>MAAQNEQRPERIKTTPYLEGDVLSSDSGPLLSVFALQEIMQKVRQVQADYMTATREVDFTVPDVQKILDDIKALAAEQVYKIVKVPSISFRHIVMQSRDRVLRVDTYYEEMSQVGDVITEDEPEKFYSTIIKKVRFIRGKGSFILHDIPTRDHRGMEVAEPEVLGVEFKNVLPVLTAEHRAMIQNALDGSIIENGNVATRDVDVFIGACSEPVYRIYNRLQGYIEAVQLQELRNSIGWLERLGHRKRITYSQEVLTDFRRQDTIWVLALQLPVNPQVVWDVPRSSIANLIMNIATCLPTGEYIAPNPRISSITLTQRITTTGPFAILTGSTPTAQQLNDVRKIYLALMFPGQIILDLKIDPGERMDPAVRMVAGVVGHLLFTAGGRFTNLTQNMARQLDIALNDYLLYMYNTRVQVNYGPTGEPLDFQIGRNQYDCNVFRADFATGTGYNGWATIDVEYREPAPYVHAQRYIRYCGIDSRELINPTTYGIGMTYHCYNEMLRMLVAAGKDSEAAYFRSMLPFHMVRFARINQIINEDLHSVFSLPDDMFNALLPDLIAGAHQNADPVVLDVSWISLWFAFNRSFEPTHRNEMLEVAPLIESVYASELSVMKVDMRHLSLMQRRFPDVLIQARPSHFWKAVLNDSPEAVKAVMNLSHSHNFINIRDMMRWVMLPSLQPSLKLALEEEAWAAANDFEDLMLTDQVYMHRDMLPEPRLDDIERFRQEGFYYTNMLEAPPEIDRVVQYTYEIARLQANMGQFRAALRRIMDDDDWVRFGGVLRTVRVKFYDARPPDDVLQGLPFSYDTNERGGLAYATIKYATETTIFYLIYNVEFSNTPDSLVLINPTYTMTKVFINKRIVERVRVGQILAVLNRRFVAYKGKMRIMDITQSLKMGTKLAAPTV[10x];> MVAITVQGAQLIKRVVERFYPGIAFNINEGACYIYKFSDHIRRIRMKHGTKYRRQAEEIIRNISLRKERLYGIPVLDEVEWKYVFDGQTFQSYAFEVYVNSILPWSELDPEEEFLRNYRVSREMTEVEKFIEFRAKNEMQIYGDIPIKVWCCFINELSAELKHVPLGMQVMADFVNRFDSPFHQGNRDLSNLEDFQVAYTTPLLFEMCCMESILEFNIKMRMREEEISALEFGDMKVDPVGLLREFFILCLPHPKKINNVLRAPYSWFVKMWGVGADPIVVLQSTAGDDRNSKDVFYDKFRT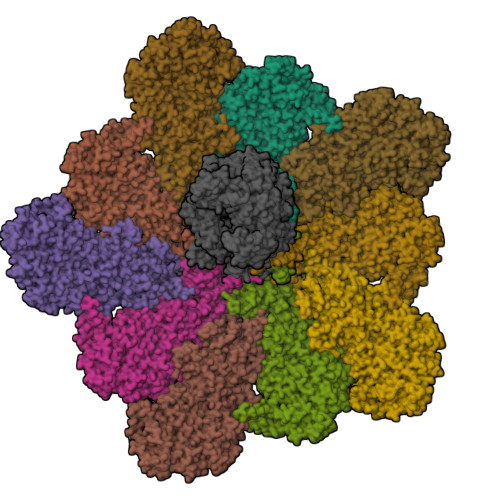EPNRYKALFRSSFYNESRRMNEEKILEAVKYSQKLGSHDRRLPLFEKMLKTVYTTPFYPHKSSNMILASFLLSIQTITGYGRAWVKNVSTEFDKQLKPNPSNLVQDVSDLTREFFKQAYVEAKERREEIVKPEDLYTSMLRLARNTSSGFSTEIYVKKRFGPRLRDKDLIKINSRIKALVIFTKGHTVFTDEELHKKYNSVELYQTKGSRDVPIKATRTIYSINLSVLVPQLIVTLPLNEYFSRVGGITSPDYKKIGGKVIVGDLEATGSRVMDAADCFRNSADRDIFTIAIDYSEYDTHLTRHNFRTGMLQGIREAMAPYRDLRYEGYTLEQIIDFGYGEGRVANTLWNGKRRLFKTTFDAYIRLDESERDKGSFKVPKGVLPVSSVDVANRIAVDKGFDTLIAATDGSDLALIDTHLSGENSTLIANSMHNMAIGTLMQREVGREQPGVLTFLSEQYVGDDTLFYTKLHTTDTKVFDKVAASIFDTVAKCGHEASPSKTMMTPYSVEKTQTHAKQGCYVPQDRMMIISSERRKDIEDVQGYVRSQVQTMITKVSRGFCHDLAQLILMLKTTFIGAWKMKRTIKEDAMYRDRKFDSNDEDGFTLIQIRNPLALYVPIGWNGYGAHPAALNIVMTEEMYVDSIMISKLDEIMAPIRRIVHDIPPCWNETQGDKRGLISATKMSFFSKMARPAVQAALSDPQIINLVEELPLGEFSPGRISRTMMHSALLKESSARTLLSSGYELEYQKALNSWITQVSMRLGEESGVISTSYAKLFDVYFEGELDGAPHMFPDQNLSPQFYIQKMMIGPRVSSRVRNSYVDRIDVILRKDVVMRGFITANTILNVIEKLGTNHSVGDLVTVFTLMNIETRVAEELAEYMTSEKIRFDALKLLKKGIAGDEFTMSLNVATQDFIDTYLAYPYQLTKTEVDAISLYCTQMIMLRAALGLPKKKMKIVVTDDAKKRYKIRLQRFRTHVPKIKVLKKLIDPNRMTVRNLENQFV> LTFEHW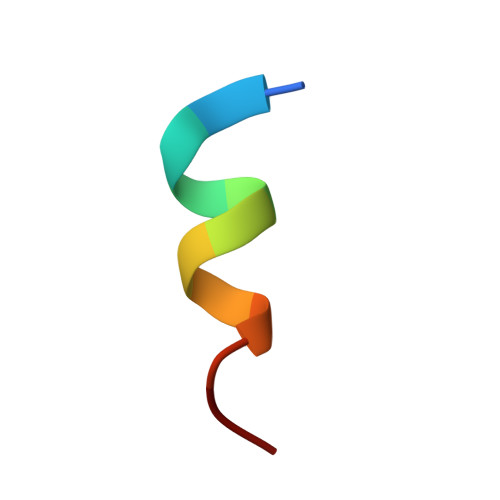WAQLTS> AECA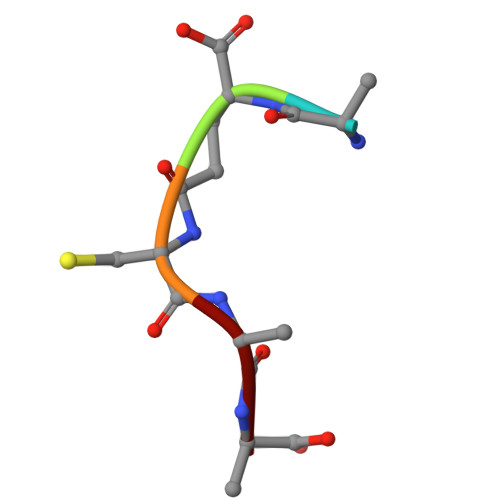A>[2x]GFLHVGKMGFVVTMLKLIQKKLLDKTCDQVMEFSWSALWNITDETPDNCEMFLNFNGMKLFLDCLKEFPEKQELHRNMLGLLGNVAEVKELRPQLMTSQFISVFSNLLESKADGIEVSYNACGVLSHIMFDGPEAWGVCEPQREEVEERMWAAIQSWDINSRRNINYRSFEPILRLLPQGISPVSQH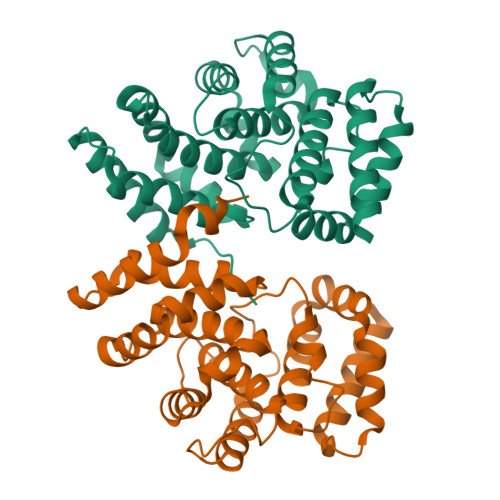WATWALYNLVSVYPDKYCPLLIKEGGMPLLRDIIKMATARQETKEMARKVIEHCSNFKEENMDTSR> MDFGSLETVVANSAFIAARGSFDASSGPASRDRKYLARLKLPPLSKCEALRESLDLGFEGMCLEQPIGKRLFQQFLRTHEQHGPALQLWKDIEDYDTADDALRPQKAQALRAAYLEPQAQLFCSFLDAETVARARAGAGDGLFQPLLRAVLAHLGQAPFQEFLDSLYFLRFLQWKWLEAQPMGEDWFLDFRVLGRGGFGEVFACQMKATGKLYACKKLNKKR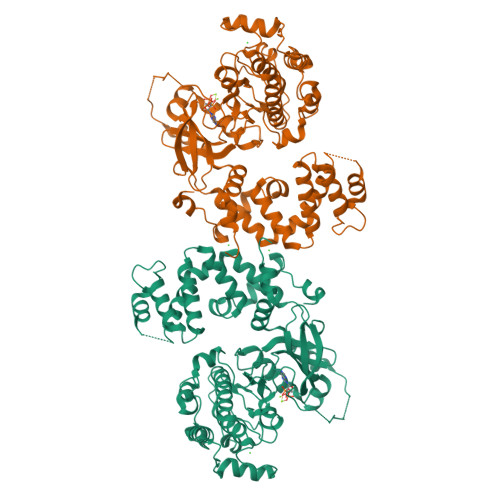LKKRKGYQGAMVEKKILAKVHSRFIVSLAYAFETKTDLCLVMTIMNGGDIRYHIYNVDEDNPGFQEPRAIFYTAQIVSGLEHLHQRNIIYRDLKPENVLLDDDGNVRISDLGLAVELKAGQTKTKGYAGTPGFMAPELLLGEEYDFSVDYFALGVTLYEMIAARGPFRARGEKVENKELKQRVLEQAVTYPDKFSPASKDFCEALLQKDPEKRLGFRDGSCDGLRTHPLFRDISWRQLEAGMLTPPFVPDSRTVYAKNIQDVGAFSTVKGVAFEKADTEFFQEFASGTCPIPWQEEMIETGVFGDLNVWRPDGVDHHHHHH>[6x]SQIPASEQETLVRPKPLLLKLLKSVGAQKDTYTMKEVLFY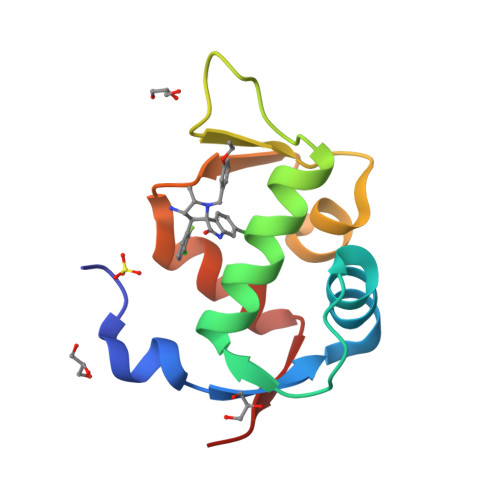LGQYIMTKRLYDEKQQHIVYCSNDLLGDLFGVPSFSVKEHRKIYTMIYRNLVVVN>[2x]RDSGTVWGALGHGINLNIPNFQMTDDI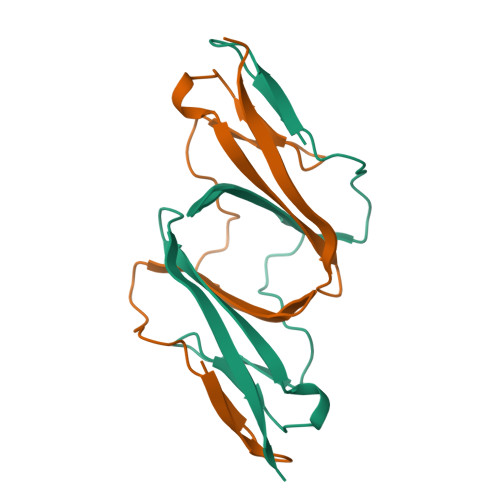DEVRWERGSTLVAEFKRKMKPFLKSGAFEILANGDLKIKNLTRDDSGTYNVTVYSTNGTRILDKALDLRILE> ASMTGGQQMGRGSSLTACPEESPLLVGPMLIE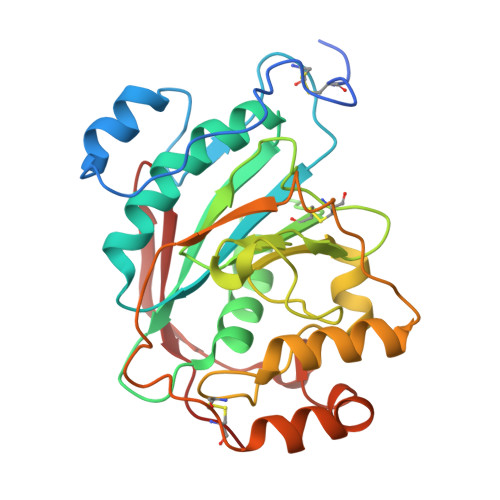FNIPVDLKLVEQQNPKVKLGGRYTPMDCISPHKVAIIIPFRNRQEHLKYWLYYLHPILQRQQLDYGIYVINQAGESMFNRAKLLNVGFKEALKDYDYNCFVFSDVDLIPMNDHNTYRCFSQPRHISVAMDKFGFSLPYVQYFGGVSALSKQQFLSINGFPNNYCGWGGEDDDIYNRLAFRGMSVSRPNAVIGKTRMIRHSRDKKNEPNPQRFDRIAHTKETMLSDGLNSLTYMVLEVQRYPLYTKITVDIGTCS>[2x]QNPADSPHIGKVFFSTNQGDFVCSANIVASANQSTVATAGHCLHDGNGGQFARNFVFAPAYDYGESEHGVWAAEELVTSAEWANRGDFEHDYAFAVLE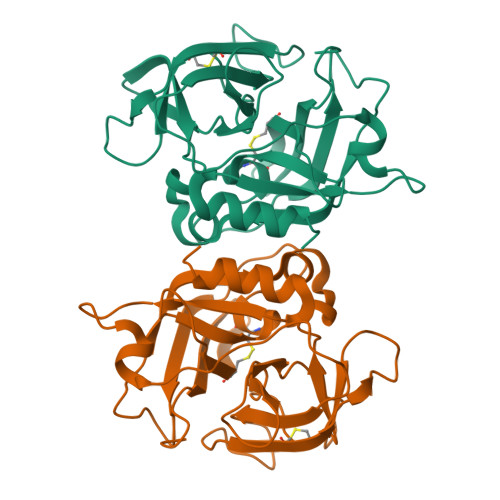TKGGTTVQQQVGTASPIAFNQPRGQYYSAYGYPAAAPFNGQELHSCHGTATNDPMGSSTQGIPCNMTGGSSGGPWFLGNGTGGAQNSTNSYGYTFLPNVMFGPYFGSGAQQNYNYASTTN> GSMVEATAQETDRPRFSFSIAAREGKARTGTIEMKRGVIRTPAFMPVGTAATVKALKPETVRATGADIILGNTYHLMLRPGAERIAKLGGLHSFMGWDRPILTDSGGYQVMSLSSLTKQSEEGVTFKSHLDGSRHMLSPERSIEIQHLLGSDIVMAFDESTPYPATPSRAASSMERSMRWAKRSRDAFDSRKEQAENAALFGIQQGSVFENLRQQSADALAEIGFDGYAVGGLAVGEGQDEMFRVLDFSVPMLPDDKPHYLMGVGKPDDIVGAVERGID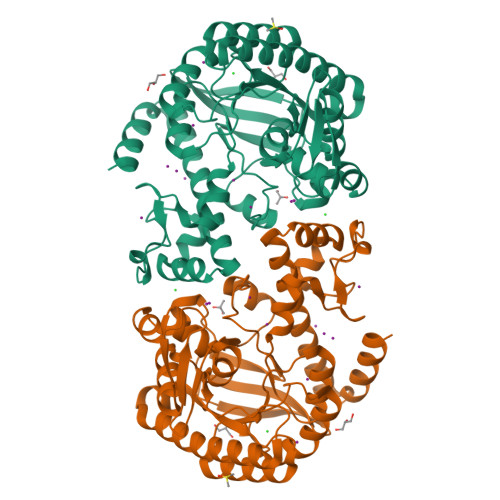MFDSVLPTRSGRNGQAFTWDGPINIRNARFSEDLKPLDSECHCAVCQKESRAYIHHLIRAGQILGAMLMTEHNIAFYQQLMQKIRDSISEGRFSQFAQDFRARYFARNS> GPETISLHR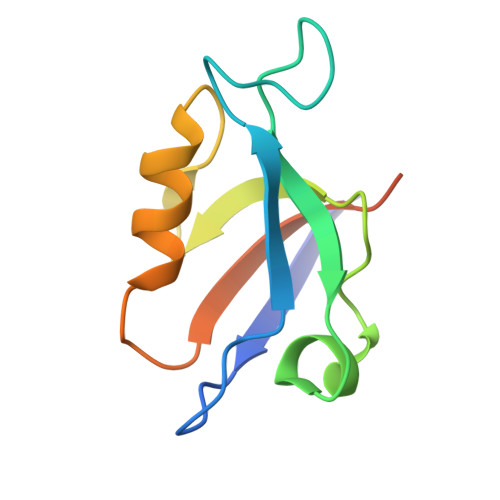QHGRGLGFTIAGGQGSPHIAGDDGIFISKIIPDSAAKEDGRLAVGDRVLSVQGESCEKITHERAVEMLRNPASPIVLVVEHNAFHKATAELSR Here, we report the discovery of potent boron-based compounds that inhibit an unprecedented target of Wolbachia, leucyl-tRNA synthetase (LeuRS), and demonstrate that inhibition of this microbiota target is an efficient approach to arrest the growth of its host. The editing site of LeuRS plays a key role to maintain fidelity in protein translation by hydrolyzing tRNALeu mischarged to noncognate amino acids such as norvaline. Altogether, these experiments show that benzoxaborole inhibitors of Wolbachia LeuRS are prodrugs that, in an enzyme-independent manner, form adducts with adenosine substrates. The adducts then bind with potent nanomolar affinity into the Wolbachia LeuRS editing site and efficiently compete with the physiological substrate norvaline.

To unveil the structural details of the inhibition mechanism of Wolbachia LeuRS by these compounds, we performed crystallization trials with the protein in the presence and absence of inhibitors and AMP. The architecture of Wolbachia LeuRS consists of six antiparallel β strands that form an extended β sheet with four inserted α helices, hence adopting a β1-β2-β3-α1-α2-β4-β5-β6-α3-α4 fold. (B) Crystal structure of Wolbachia LeuRS D1 editing domain shown in cartoon representation with key secondary elements colored as in (A). In addition, the region 313 to 318, which, as judged by the high crystallographic B factors, is highly flexible in the apo-structure, becomes more compact in the complex and makes interactions to the adduct. The new high-resolution crystal structures presented reveal idiosyncratic features at the drug binding pocket, which rationalize the selectivity of these Wolbachia inhibitors.

>GAMGKSEGVTIEFKIVGLNKKLKVFTTCPHTLFGASFCAVAIEHPIVQDLMSKEIQDLISSIKIQGKNNEKVGIYTGLNVKHPFLDKELPLYVANFVLMEYREGAIFGCPAHDQRDFEFAQEYDLPIIPVISSARLGIEEYTNNSIMFNSEFLNGLTVSEARKVIVEKLEEKGIGKKTI[4x]>MSKTRVIYPGTFDPITNGHVDLVTRASRMFDEVVVAIAIGHHKNPLFSLEERVALAQSSLGHLSNVEFVGFDGLLVNFFKEQKATAVLRGLRAVSDFEYEFQLANMNRQLDPHFEAVFLTPSEQYSFISSTLIREIARLKGDVTKFVPQAVVEAFERKHQQGW[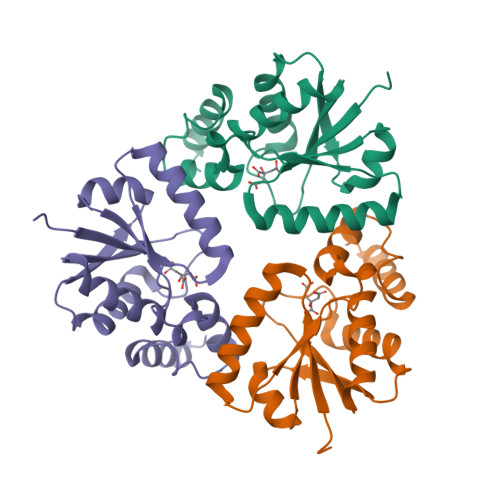3x]>[44x]MALNSINTNSGALIALQNLNSTNAELTQVQQRINTGKKIGSAKDNGAIWATAKNQSATAGSMNAVKDSLQRGQSTIDVALAAGDTITD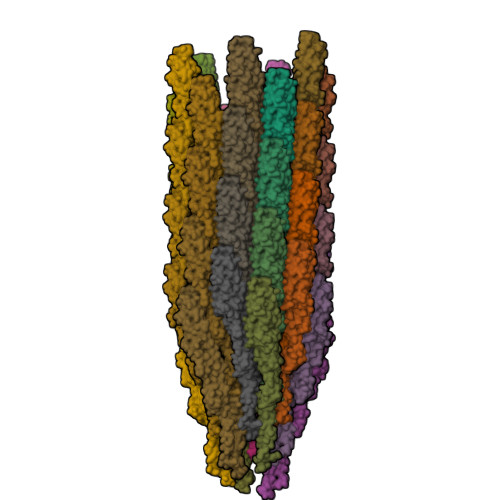LLGKMKEKALAASDTSLNTASFNALKSDFDSLRDQITKAASNAKFNGVSIADGTTTKLSFLANSDGSAFTVTAKTLTLGGLGLTATSSFTTAAAAKTMIGTIDTALQTATNKLASLGTSSTGLDTHLTFVGKLQDSLDAGVGNLVDADLAKESAKLQSLQTKQQLGVQALSIANQSSSSILSLFR> MVLPRKLVGQCCLLLQKKQTAASYMANAGKVGNEEKWAQAAMEYLHEKRHCNDSRKRQHDVDNERRMAFAFDRYCSVNEKIFTERLSRLSDRMTEALETIKQLGMDHALEE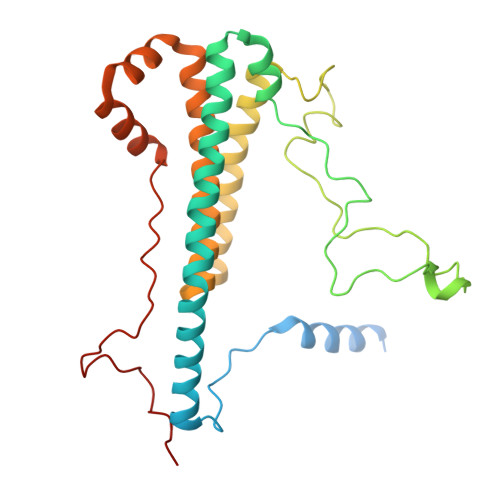ALMLSSEQPPLNFRRPTLTPPVAGYEPGFGLDVPQLRSRQAEYPPVGRPTDAMEFGEEKDPSFPLVESFRVEDLTTQCLNELEERHGEIREAAPTTGVEGEAWEAYVALQKKALARQQLIFELCNNGELRERYDSDVAFRQRVWEERGMLPLEIERERLHEEPRHYAQEPAYHPFRKM> MGHHHHHHHHHHSSGHIEGRHMEANGLGPQGFPELKNDTFLRAAWGEETDYTPVWCMRQAGRYLPEFRETRAAQDFFSTCRSPEACCELTLQPLRRFPLDAAIIFSDILV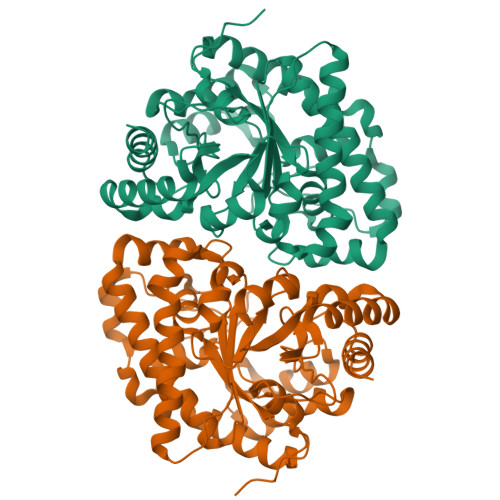VPQALGMEVTMVPGKGPSFPEPLREEQDLERLRDPEVVASELGYVFQAITLTRQRLAGRVPLIGFADAPWTLMTYMVEGGGSSTMAQAKRWLYQRPQASHQLLRILTDALVPYLVGQVVAGAQALQLFESHAGHLGPQLFNKFALPYIRDVAKQVKARLREAGLAPVPMIIFAKDGHFALEELAQAGYEVVGLDWTVAPKKARECVGKTVTLQGNLDPCALYASEEEIGQLVKQMLDDFGPHRYIANLGHGLYPDMDPEHVGAFVDAVHKHSRLLRQN1-(2-methyl-1,3-benzoxazol-6-yl)-3-(1,5-naphthyridin-4-yl)urea 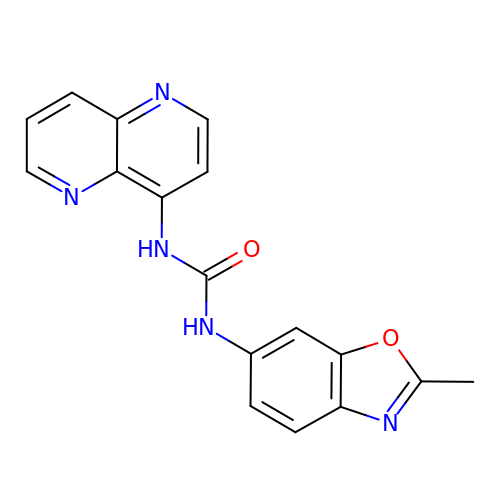| C17 H13 N5 O2 | AKMNUCBQGHFICM-UHFFFAOYSA-N>[2x]MTDFTPETPVLTPIRDHAAELAKAEAGVAEMAAKRNNRWYPKYHIASNGGWI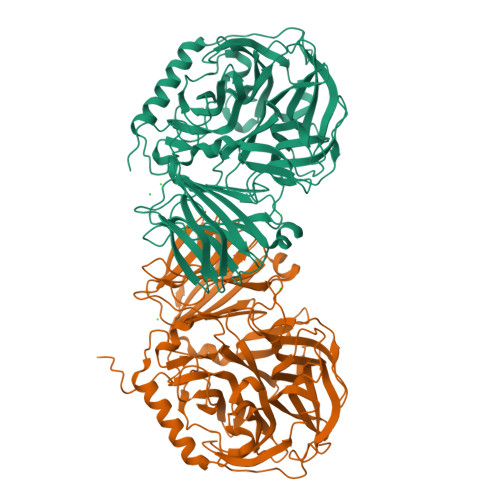NDPNGLCFYKGRWHVFYQLHPYGTQWGPMHWGHVSSTDMLNWKREPIMFAPSLEQEKDGVFSGSAVIDDNGDLRFYYTGHRWANGHDNTGGDWQVQMTALPDNDELTSATKQGMIIDCPTDKVDHHYRDPKVWKTGDTWYMTFGVSSADKRGQMWLFSSKDMVRWEYERVLFQHPDPDVFMLECPDFSPIKDKDGNEKWVIGFSAMGSKPSGFMNRNVSNAGYMIGTWEPGGEFKPETEFRLWDCGHNYYAPQSFNVDGRQIVYGWMSPFVQPIPMEDDGWCGQLTLPREITLGDDGDVVTAPVAEMEGLREDTLDHGSVTLDMDGEQIIADDAEAVEIEMTIDLAASTAERAGLKIHATEDGAYTYVAYDGQIGRVVVDRQAMANGDRGYRAAPLTDAELASGKLDLRVFVDRGSVEVYVNGGHQVLSSYSYASEGPRAIKLVAESGSLKVDSLKLHHMKSIGLELEHHHHHH>GPDSENGVGDAELRERLRQCEETIEQLRAENQELKRKLNILTRPSGILVNDTKLDGPILQILFMNNAISKQYHQEIEEFVSNLVKRFEEQQKNDVEKTSFNLLPQPSSIVLEEDHKVEESCAIKNNKEAFSVVGSVLYFTNFCLDKLGQPLLNENPQLSEGWEIPKYHQVFSHIVSLEGQEIQVKAKRPKPHCFNCGSEEHQMKDCPMPRNAARISEKRKEYMDACGEANNQNFQQRYHAEEVEERFGRFKPGVISEELQDALGVTDKSLPPFIYRMRQLGYPPGWLKEAELENSGLALYD[2x];>GPDSMADAFGDELFSVFEGDSTTAAGTKKDKEKDKGKWKGPPGSADKAGKRFDGKLQSESTNNGKNKRDVDFEGTDEPIFGKKPRIEESITEDLSLADLMPRVKVQSVETVEGCTHEVALPAEEDYLPLKPRVGKAAKEYPFILDAFQREAIQCVDNNQSVLVSAHTSAGKTVCAEYAIALALREKQRVIFTSPIKALSNQKYREMYEEFQDVGLMTGDVTINPTASCLVMTTEILRSMLYRGSEVMREVAWVIFDEIHYMRDSERGVVWEETIILLPDNVHYVFLSATIPNARQFAEWICHLHKQPCHVIYTDYRPTPLQHYIFPAGGDGLHLVVDENGDFREDNFNTAMQVLRDAGDLAKGDQKGRKGGTKGPSNVFKIVKMIMERNFQPVIIFSFSKKDCEAYALQMTKLDFNTDEEKKMVEEVFSNAIDCLSDEDKKLPQVEHVLPLLKRGIGIHHGGLLPILKETIEILFSEGLIKALFATETFAMGINMPARTVLFTNARKFDGKDFRWISSGEYIQMSGRAGRRGMDDRGIVILMVDEKMSPTIGKQLLKGSADPLNSAFHLTYNMVLNLLRVEEINPEYMLEKSFYQFQHYRAIPGVVEKVKNSEEQYNKIVIPNEESVVIYYKIRQQLAKLGKEIEEYIHKPKYCLPFLQPGRLVKVKNEGDDFGWGVVVNFSKKSNVKPNSGELDPLYVVEVLLRCSKESLKNSATEAAKPAKPDEKGEMQVVPVLVHLLSAISSVRLYIPKDLRPVDNRQSVLKSIQEVQKRFPDGIPLLDPIDDMGIQDQGLKKVIQKVEAFEHRMYSHPLHNDPNLETVYTLCEKKAQIAIDIKSAKRELKKARTVLQMDELKCRKRVLRRLGFATSSDVIEMKGRVACEISSADELLLTEMMFNGLFNDLSAEQATALLSCFVFQENSSEMPKLTEQ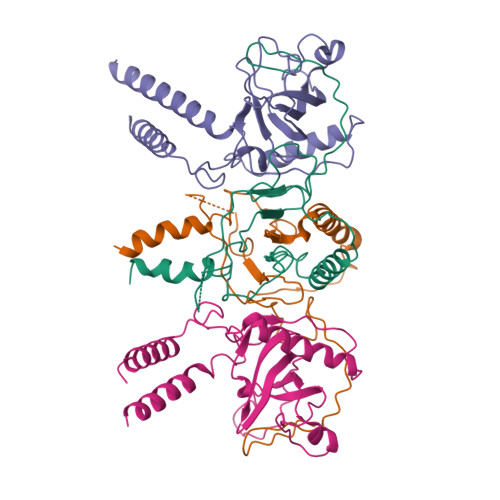LAGPLRQMQECAKRIAKVSAEAKLEIDEETYLSSFKPHLMDVVYTWATGATFAHICKMTDVFEGSIIRCMRRLEELLRQMCQAAKAIGNTELENKFAEGITKIKRDIVFAASLYL[2x]>[2x]FQSMDLPDIVNMYFDADSCND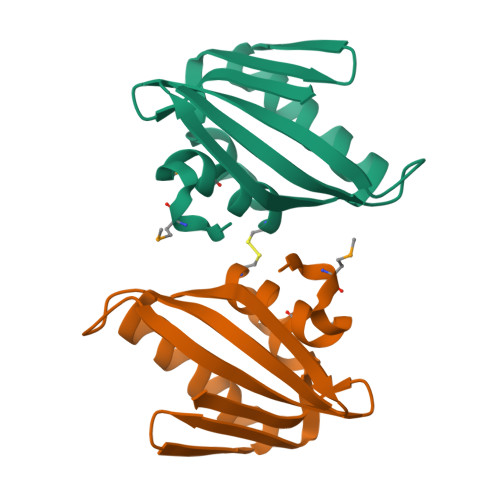TDALSETFAPDAVVEDEGARHQGVVAILRWWVAAKKAASYVAEPLESTVDGDKALVRAKVSGRFPGSPVTLTYSFTIKDGRIARLEIQ> MPVITVNTNVAEKSIPVFFQAALTNMMTKALQKPKEVMFVDLRSGANIMMGGDRNPCVFATVECIGRLNPTSNLAMARDMEDMFIEHLNVRRERIVIRFIPVPALFCSFNGALHDVSIERDEDIISQAIAEYLAAHAA;> MPVITVNTNVAEKSIPVFFQAALTNMMTKALQKPKEVMFVDLRSGANIMMGGDRNPCVFATVECIGRLNPTSNLAMARDMEDMFIEHLNVRRERIVIRFIPVPALFCSFNGALHDVSIERDEDIISQAIAEYLHHHHHHH;> MPV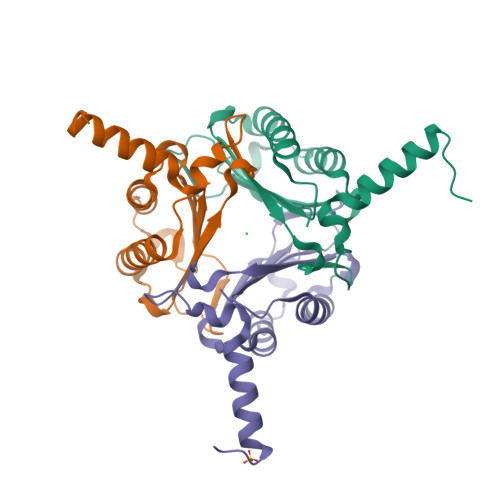ITVNTNVAEKSIPVFFQAALTNMMTKALQKPKEVMFVDLRSGANIMMGGDRNPCVFATVECIGRLNPTSNLAMARDMEDMFIEHLNVRRERIVIRFIPVPALFCSFNGALHDVSIERDEDIISQAIAEYLHHHHH;> MPVITVNTNVAEKSIPVFFQAALTNMMTKALQKPKEVMFVDLRSGANIMMGGDRNPCVFATVECIGRLNPTSNLAMARDMEDMFIEHLNVRRERIVIRFIPVPALFCSFNGALHDVSIERDEDIISQAIAEYLHHHHHHHA> GSTMSLSRSEEMHRLTENVYKTIMEQFNPSLRNFIAMGKNYEKALAGVTYAAKGYFDALVKMGELASESQGSKELGDVLFQMAEVHRQIQNQLEEMLKSFHNELLTQLEQKVELDSRYLSAALKKYQTEQRSKGDALDKCQAELKKLRKKSQGSKNPQKYSDKELQYIDAISNKQGELENYVSDGYKTALTEERRRFCFLVEKQCAVAKNSAAYHSKGKELLAQKLPLWQQACADPSKIPERAVQLM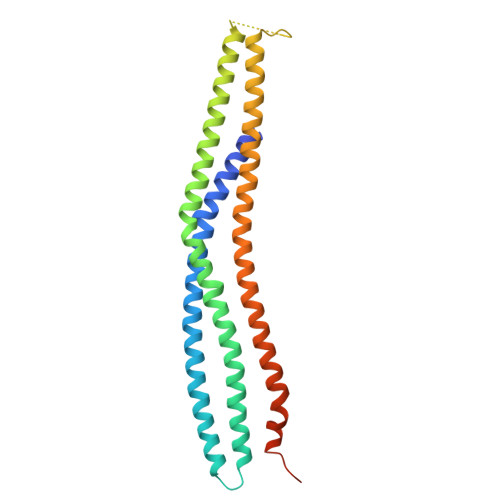QQVASN SERINE-3'-AMINOADENOSINE 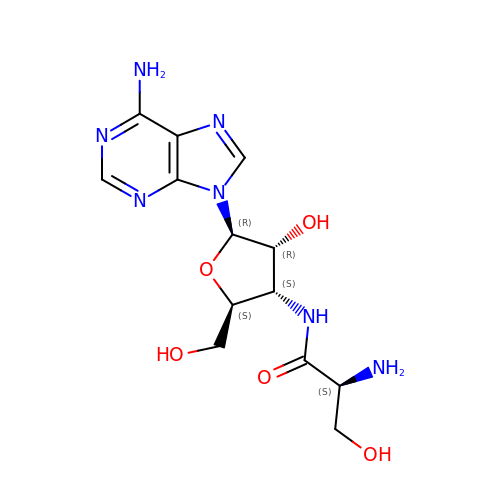| C13 H19 N7 O5 | ITDKSTILAWHDJI-AYEBZEFBSA-N RNA helicase DDX21 plays vital roles in ribosomal RNA biogenesis, transcription, and the regulation of host innate immunity during virus infection. DDX21 is composed of three domains, including the N‐terminal domain, the middle D1 and D2 domain, and the C‐terminal foldase domain. In summary, here we reported multiple sets of crystal structures of RNA helicase DDX21 either in ligand‐free (DDX21‐apo) or in complex with AMP (DDX21‐AMP), ADP (DDX21‐ADP), or a nonhydrolyzable ATP analog (AMPPNP) and a 15‐nucleotide poly(U) ssRNA (DDX21‐AMPPNP‐U15), corresponding to different unwinding states (except for DDX21‐AMP). We elucidated the conformational rearrangements upon the ATP and ssRNA binding during the dsRNA unwinding cycle, and described an RNA unwinding machinery including one wedge helix, one sensor motif V, and the DEVD box.

Moreover, crystal structure of DDX21 with an ADP molecule was solved at 2.7 Å; however, one internal loop was disordered (residues Ile400 – Ile409), and the ADP molecule for crystallization was spontaneously hydrolyzed into AMP. Further SDS‐PAGE analysis of the DDX21‐AMP crystals indicated that the missing loop was degraded. While in AMPPNP, ADP, or AMP bound states, the “TG loop” was open, and therefore accommodated ligand binding.

>SFSNFPISEETIKLLKGRGVTFLFPIQAKTFHHVYSGKDLIAQARTGTGKTFSFAIPLIEKLHGELQDRKRGRAPQVLVLAPTRELANQVSKDFSDITKKLSVACFYGGTPYGGQFERMRNGIDILVGTPGRIKDHIQNGKLDLTKLKHVVLDEVDQMLDMGFADQVEEILSVAYKKDSEDNPQTLLFSATCPHWVFNVAKKYMKSTYEQVDLIGKKTQKTAITVEHLAIKCHWTQRAAVIGDVIRVYSGHQGRTIIFCETKKEAQELSQNSAIKQDAQSLHGDIPQKQREITLKGFRNGSFGVLVATNVAARGLDIPEVDLVIQSSPPKDVESYIHRSGRTGRAGRTGVCICFYQHKEEYQLVQVEQKAGIKFKRI[5x]> XKETA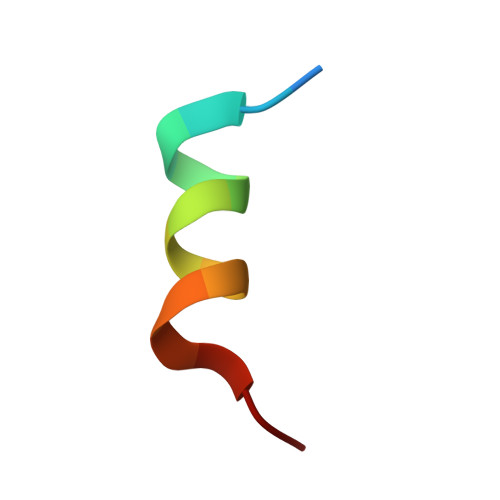AXKFEXQHMDS>[2x]MVESDSSGIVRHSQGEFDIVQVYKKFLQDDPEITMPVAAIEALVQLLSRSQAKTISEFMDILQNGSNTLKEGVQNNISLSAGCDIFQRFVTRSLHDVGDFEQCKRHLVENGKLFIQRARACRQRIAHLGYPLIRDGSVILTHGFSRGVAAVLLAAAKRHVRFKVFVTESRPSGSGCLMTRTLKNACIPTCMVLDSAVSFTMNRVDLVLVGAEGVVENGGLINQIGTFQLAVFAKHAHKPFYAVAESHKFVRMFPLSQYDIPFSRPILEFDDPSPETVHPEPEPIPTPSDAIHNELIMNEEQIRNNPTLDVTPPEFVSGLITDLGIIDSKSGVSEELIKLYL;>[2x]GPISEFMSTINVEHTYPAVSSLIADLKSRKVQGPFAVAVETALVMRQVISQTRWSTVDQLIDTVRAVGSTLVKAQPTEFSCGNIIRRILRLIREEYQELLKTADENEKLIVSSSNSSSPSQKRDIPSNEKLVQSHEPVSVQMYSSMLNLLGRPTLESPTHSKTVGDSRVTGGMDMRAVIISGIQDVIDELDKINTDIEVQSMDHLHSNEIILTQGCSKTVEAFLRFAAKKRKFSVIVAEGFPNNQKGSHAMAKRLAQAGIDTTVISDATIFAIMSRVNKVILGTHAILGNGGLVTYSGAQLVAQAARHHATPVVVCSGIYKLSPVYPYDLESIIQLSSPDKIMSFNEGDLISRAEILNPYYDYIPPDLVDLFITNLGGYPPSYLYRIMNDTYDASDTIL;>[2x]MSLYEHAALPLASSPSILGPISGGRNRGNIQLQSIPIEFQAVVFAGFGNSLYPLTGSDALPKALLPIGNKPMLHYPLYWLEAAGFTSAILICMEEAEAHINAWLRSGYEGHMRIHVEAPTILDDSKSSADALRAVSHLIKNDFVCLSCDSIVGLPPYTVLDKFRLDNPSALAVYSPVLKYEHITSQSKEIDAKQLIGIEEKTSRLLYAKSSADVGSDFTFRMSLLWKHPRVTLNTNLSDAHIFVFKHWVIDLIREKESISSIRGDLIPYLVKCQYQKSFTVRENIQRFLSSPNNIDNYDGGLSSQEIKINALIAKDGIICSRANNLPNYFELNKCIAKLTPEQRLVDVTVSERALVGADCMVNEGTTIKDNSNIKKSIIGKNCVIGKGVVVSNSILMDNIVVEDGVRLESCIVASGAQIGAKSKLRECEIGVDHRVEAGRIARGERLVDMEKIETDMD;>MGFSAEQAKKDGKDQSPVSESSSVGGTSPATASSVVSPNEPKLSGKEAKALKKARKQASRRAKAEAAAANNPPGVSEEKKVAIPNKNSNQQKKASKQNPQNSPETDANLQEKKIFEEKQVSIFSHLDWRRRRTTENIPKDIHPAVIRLGLKLANYKIFGSNQRCIDLLKTFKIVIQDYQTPYGTTLSRHLTTHINSQIAYLVSTRPLSISMGNAIRFLKLEISVLDIDLTDDEGKELLLEKIDSYIRDRIIIAGQVIVQAATEKIQDGDVILTYLHSSTVNDVLIHAKNVGKKFRVVVVDSRPEFEGRVCLKLLTEHGIECTYVMISALSYIMQEVTKIFLGGHAMLSNGALYSRAGTSLISLLGHESNVPVIACCESYKFTERIQLDSLVYNELAPGDQLVNMGVDDFEEKPGVLANWKSVKNLKLLSLKYDVTPPRLITVC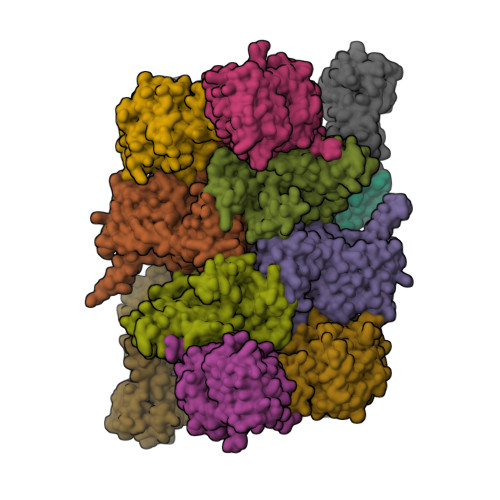VCEMGLLPSTSVPAIINEFKQVYA[2x];>[2x]MPPSKGLNGKLEKPKHALQAIVLSDSYNYRFRPLTLDKPRCLLPLANTPLIEYTFEFLALAGVQEVYVFCCAHAGQIREYIEKSKWNLPSSPFSVNTIVSRESLSVGDALRELDSKQLITSDFILVSGDVVSNVPLNEVLKEHRKRREDDKNAIMTMVVREASPFHRTRARTESSVFVIDKKTSQCVHYQANERGKHYVSMDPEIFNEHEELEVRNDLIDCQIDICSNDVPALFTENFDYQDIRKDFVYGVLTSDLLGKKIHCHVAKENYAARVRSLQTYDAISKDVLSRWVYPFVPDSNLLNQTFSYQRHQIYKEEDVVLARSCIIKARTLIGAYTKVGDASVVANTIIGRNCTIGSNCSIDSAFLWEDVVIGDNCRIGKAILANSVKIGNNCSIEDGAIVAAGVVIGDNTIIEKNKRLTTFESHSQGTLNDPSLVGIGGRGQEYHAEEDSDDEGEFMEASGLIESTNELHLSDSESSETSSSSEEDMEFIPFSARRDSANTINSEDFDEGDFNKEAQQSLERAFEENHQIDIAALELNTLRMAMNANYHEVRSAIVLALLRRIMHLDVSPKEALAKVMTRWGPLLAKLTFSHEEQVDNVLTLQKYCVRLSMTRHFLQLLGYFYQLEIAEENAIQEWYSDPRSSEGELAALRDAGGKQFVDWLNTAESESESEEGSE;>[2x]MSTSHCRFYENKYPEIDDIVMVNVQQIAEMGAYVKLLEYDNIEGMILLSELSRRRIRSIQKLIRVGKNDVAVVLRVDKEKGYIDLSKRRVSSEDIIKCEEKYQKSKTVHSILRYCAEKFQIPLEELYKTIAWPLSRKFGHAYEAFKLSIIDETVWEGIEPPSKDVLDELKNYISKRLTPQAVKIRADVEVSCFSYEGIDAIKDALKSAEDMSTEQMQVKVKLVAAPLYVLTTQALDKQKGIEQLESAIEKITEVITKYGGVCNITMPPKAVTATEDAELQALLESKELDNRSDSEDDEDESDDE> XSRA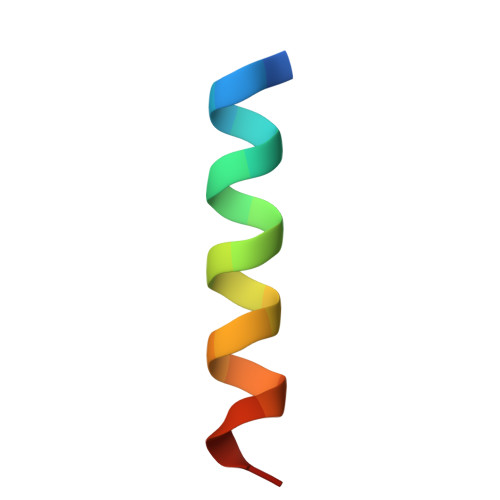QILCKATEYIQYMRRKN> QQMEGNGPAAVHYQPASPPRDACVYSSCYSEENVWKLCEYIKNHDQYPLEECYAVFISNERKMIPIWKQQARPGDGPVIWDYHVVLLHVSSGGQSFIYDLDTVLPFPCLFDTYVEDAIKSDDDIHPQFRRKFRVICADSYLKNFAS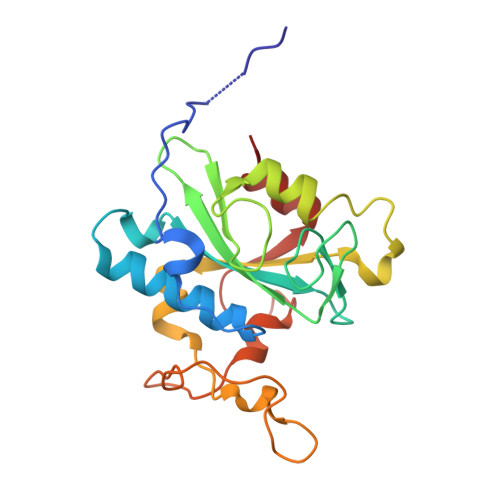DRSHMKDSSGNWREPPPPYPCIETGDSKMNLNDFISMDPKVGWGAVYTLSEFTHRFGS>[16x]WIENIPLAEEEHNKWHQDAVSLHLEFGIPRTAAEDIVQQCDVCQENKM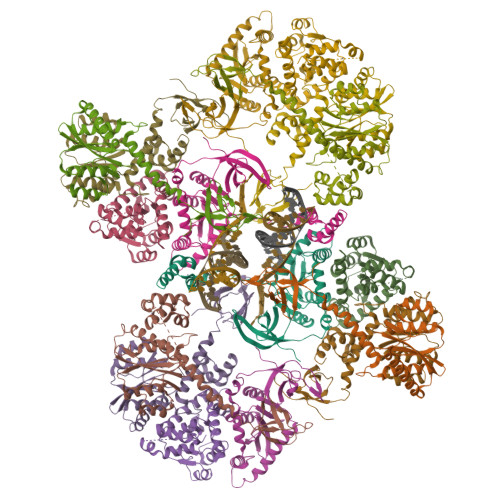PSTLRGSNKRGIDHWQVDYTHYEDKIILVWVETNSGLIYAERVKGETGQEFRVQTMKWYAMFAPKSLQSDNGPAFVAESTQLLMKYLGIEHTTGIPWNPQSQALVERTHQTLKNTLEKLIPMFNAFESALAGTLITLNIKRKGGLGTSPMDIFIFNKEQQRIQQQSKSKQEKIRFCYYRTRKRGHPGEWQGPTQVLWGGDGAIVVKDRGTDRYLVIANKDVKFIPPPKEIQKE Norrie Disease Protein (NDP) gene encodes Norrin, a secreted cystine-knot like growth factor, distinct from the lipid-modified Wnt. Unlike Wnts which have promiscuous interactions with Fz receptors, Norrin specifically binds to Fz4CRD, but not to the 14 other CRDs of Fz and secreted Frizzled-related protein (sFRP) family members. The Norrin mediated pathway maintains the blood-retina and blood-brain barriers and regulates angiogenesis in the cochlea and uterus as well as neuroprotective effects on retinal neurons. Our crystallographic and solution studies further reveal that dimeric Norrin forms a complex with two copies of monomeric Fz4CRD.

We determined three crystal structures of Norrin, using selenomethionine-labeled protein for phasing. The Norrin protein fold is identical to that of the previously reported MBP-Norrin crystal structure. Each Norrin monomer comprises three β-hairpins (β1-β2, β3-β4 and β5-β6), a β7 strand at the C-terminus, and four intramolecular disulphide bonds. The two monomers assemble as an elongated, head-to-tail, dimer stabilized by three intermolecular disulphide bridges (Cys93-Cys95, Cys95-Cys93, and Cys131-Cys131), in agreement with small-angle X-ray scattering (SAXS) measurements which showed Norrin dimer in solution. The dimer interface is further stabilized by extensive hydrogen bonds and hydrophobic interactions. Superposition of all molecules in the asymmetric units from our three crystal forms with the MBP-Norrin structure showed an average root-mean-square (r.m.s.) deviation of 1.5 Å over 190 equivalent Cα atoms. On inspection the superpositions revealed a high degree of conformational plasticity in the β1-β2, β3-β4 and β5-β6 loops. The flexibility inherent in these regions is consistent with the relatively high crystallographic B factor values. Conversely, the structural comparisons underscore the conserved nature of the interface at the dimer core.

>GPGKTDSSFIMDSDPRRCMRHHYVDSISHPLYKCSSKMVLLARCEGHCSQASRSEPLVSFSTVLKQPFRSSCHCCRPQTSKLKALRLRCSGGMRLTATYRYILSCHCEECNSGTETSQVAPA[4x]(2~{S})-~{N}-[(2~{S})-3-methoxy-1-(naphthalen-1-ylmethylamino)-1-oxidanylidene-propan-2-yl]-4-oxidanylidene-2-(3-phenylpropanoylamino)-4-piperidin-1-yl-butanamide 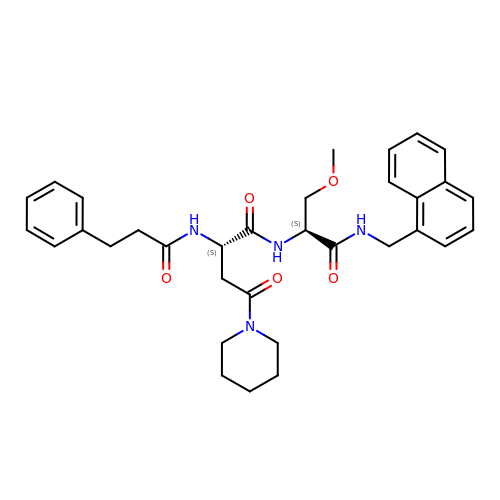| C33 H40 N4 O5 | WFBJQCJVXAHYAP-VMPREFPWSA-N>MTPSHPARPSRSGILVFDVNETLLDLTSLSPLFERVFGDAKVLREWFPELILYSQTLTLTGLYRPFGEIAAAVFEMVAANHQAKVTPDDIAELKTRLTSMPAYPDVAPALTRLQDAGFRLVTLTNSAPSPAPSPLEKAGIASFFEAHLTVHSSQRFKPHPSVYDSTAETLGA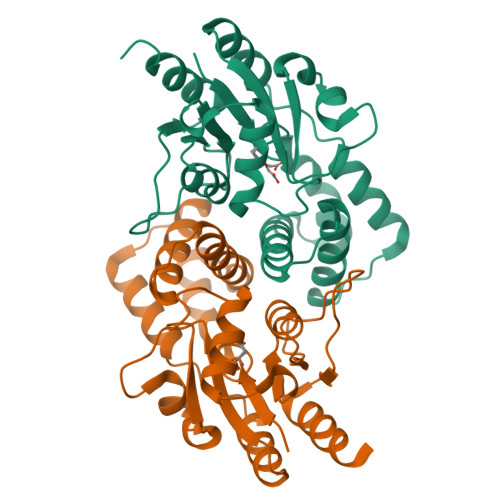KPEELCMIACHIWDTIGAQARGWRGGFVARPHNTPLTLAEVPQPDFIGRDMGELADQLIASLTA[2x]> GDPIADMIDQTVNNQVNRSLTALQVLPTAANTEASSHRLGTGVVPALQAAETGASSNASDKNLIETRCVLNHHSTQETAIGNFFSRAGLVSIITMPTTGTQNTDGYVNWDIDLMGYAQLRRKCELFTYMRFDAEFTFVVAKPNGELVPQLLQYMYVPPGAPKPTSRDSFAWQTATNPSVFVKMTDPPAQVSVPFMSPASAYQWFYDGYPTFGEHLQANDLDYGQCPNNMMGTFSIRTVGTEKSPHSITLRVYMRIKHVRAWIPRPLRNQPYLFKTNPNYKGNDIKCTSTSRDKITTL;> MGSQVSTQRSGSHENSNSASEGSTINYTTINYYKDAYAASAGRQDMSQDPKKFTDPVMDVIHEMAPPLKSPSAEACGYSDRVAQLTIGNSTITTQEAANIVIAYGEWPEYCPDTDATAVDKPTRPDVSVNRFFTLDTKSWAKDSKGWYWKFPDVLTEVGVFGQNAQFHYLYRSGFCVHVQCNASKFHQGALLVAVLPEYVLGTIAGGTGNENSHPPYATTQPGQVGAVLTHPYVLDAGIPLSQLTVCPHQWINLRTNNCATIIVPYMNTVPFDSALNHCNFGLLVIPVVPLDFNTGATSEIPITVTIAPMCAEFAGLRQAVKQ;> GIPTELKPGTNQFLTTDDGVSAPILPGFHPTPPIHIPGEVHNLLEICRVETILEVNNLKTNETTPMQRLCFPVSVQSKTGELCAAFRADPGRDGPWQSTILGQLCRYYTQWSGSLEVTFMFAGSFMATGKMLIAYTPPGGNVPADRITAMLGTHVIWDFGLQSSVTLVVPWISNTHYRAHARAGYFDYYTTGIITIWYQTNYVVPIGAPTTAYIVALAAAQDNFTMKLCKDTEDIEQTANI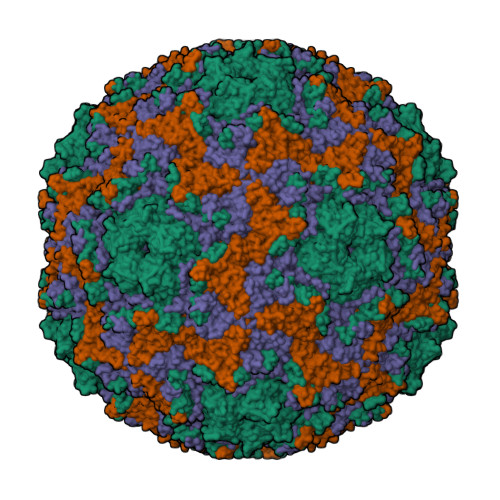Q>GDEGNIKENAVRMMECIVNKDSEKLFDFYNKDMKDNYKDS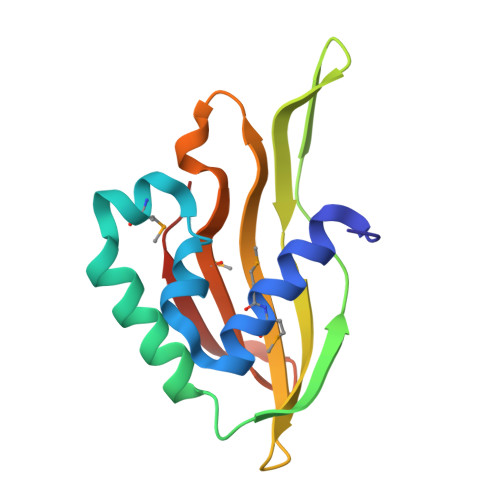SLDEIRQLFEYIDGAITSYNYEGKGGGQEAKNDGIICYYSCHPEFDFTTETGQEYTISFSYHYIWNEHPEYEGINMIQICKDGNWGEKLIIGRNYYKE[2x]> MTTFPTLDPELAAALTMLPKVDFADLPNARATYDALIGAMLADLSFDGVSLRELSAPGLDGDPEVKIRFVTPDNTAGPVPVLLWIHGGGFAIGTAESSDPFCVEVARELGFAVANVEYRLAPETTFPGPVNDCYAALLYIHAHAE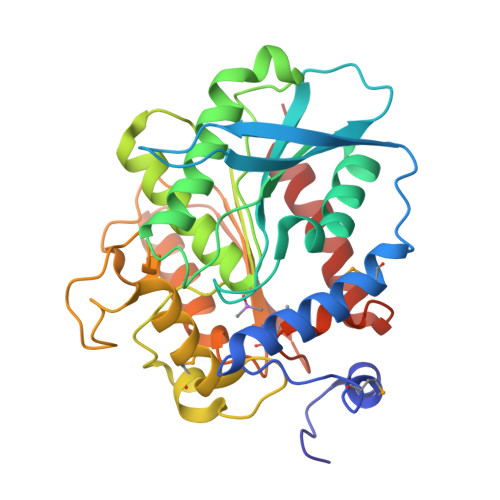ELGIDPSRIAVGGQSAGGGLAAGTVLKARDEGVVPVAFQFLEIPELDDRLETVSMTNFVDTPLWHRPNAILSWKYYLGESYSGPEDPDVSIYAAPSRATDLTGLPPTYLSTMELDPLRDEGIEYALRLLQAGVSVELHSFPGTFHGSALVATAAVSERGAAEALTAIRRGLRSLSPVS> MNLLIDNWIPVRPRNGGKVQIINLQSLYCSRDQWRLSLPRDDMELAALALLVCIGQIIAPAKDDVEFRHRIMNPLTEDEFQQLIAPWIDMFYLNHAEHPFMQTKGVKANDVTPMEKLLAGVSGATNCAFVNQPGQGEALCGGCTAIALFNQANQAPGFGGGFKSGLRGGTPVTTFVRGIDLRSTVLLNVLTLPRLQKQFPNESHTENQPTWIKPIKSNESIPASSIGFVRGLFWQPAHIELCDPIGIGKCSCCGQESNLRYTGFLKEKFTFTVNGLWPHPHSPCLVTVKKGEVEEKFLAFTTSAPSWTQISRVVVDKIIQNENGNRVAAVVNQFRNIAPQSPLELIMGGYRNNQASILERRHDVLMFNQGWQQYGNVINEIVTVGLGYKTALRKALYTFAEGFKNKDFKGAGVSVHETAERHFYRQSELLIPDVLANVNFSQADEVIADLRDKLHQLCEMLFNQSVAPYAHHPKLISTLALARATLYKHLRELKPQGGPSNG;>GPGYQMADEIDAMALYRAWQQLDNGSCAQIRRVSEPDELRDIPAFYRLVQPFGWENPRHQQALLRMVFCLSAGKNVIRHQDKKSEQTTGISLGRALANSGRINERRIFQLIRADRTADMVQLRRLLTHAEPVLDWPLMARMLTWWGKRERQQLLEDFVLTTNKNA[2x];>[6x]MSNFINIHVLISHSPSCLNRDDMNMQKDAIFGGKRRVRISSQSLKRAMRKSGYYAQNIGESSLRTIHLAQLRDVLRQKLGERFDQKIIDKTLALLSGKSVDEAEKISADAVTPWVVGEIAWFCEQVAKAEADNLDDKKLLKVLKEDIAAIRVNLQQGVDIALSGRMATSGMMTELGKVDGAMSIAHAITTHQVDSDIDWFTAVDDLQEQGSAHLGTQEFSSGVFYRYANINLAQLQENLGGASREQALEIATHVVHMLATEVPGAKQRTYAAFNPADMVMVNFSDMPLSMANAFEKAVKAKDGFLQPSIQAFNQYWDRVANGYGLNGAAAQFSLSDVDPITAQVKQMPTLEQLKSWVRNNGEA;> MRSYLILRLAGPMQAWGQPTFEGTRPTGRFPTRSGLLGLLGACLGIQRDDTSSLQALSESVQFAVRCDELILDDRRVSVTGLRDYHTVLGAREDYRGLKSHETIQTWREYLCDASFTVALWLTPHATMVISELEKAVLKPRYTPYLGRRSCPLTHPLFLGTCQASDPQKALLNYEPVGGDIYSEESVTGHHLKFTARDEPMITLPRQFASREWYVIKGGMDVSQ;> MYLSKVIIARAWSRDLYQLHQGLWHLFPNRPDAARDFLFHVEKRNTPEGCHVLLQSAQMPVSTAVATVIKTKQVEFQLQVGVPLYFRLRANPIKTILDNQKRLDSKGNIKRCRVPLIKEAEQIAWLQRKLGNAARVEDVHPISERPQYFSGDGKSGKIQTVCFEGVLTINDAPALIDLVQQGIGPAKSMGCGL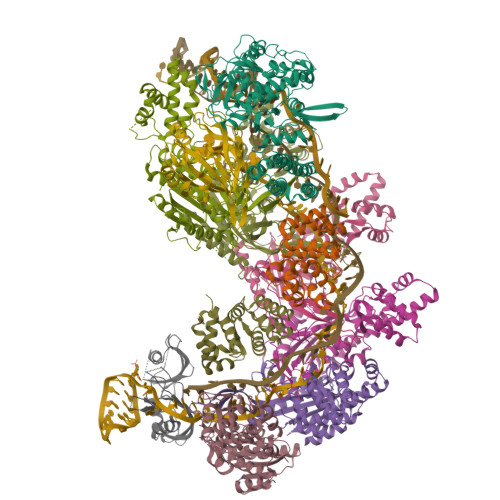LSLAPL>[2x]MNYWWVSQKQTFKQEFEGGYMWSPKENKNGTQSHYYNNMTLVQPGDVVFSFANGLILSVGIARSHAYSYNKPTEFGVAGADWANDGWKIDLEYHLVENKIRPKAHIDFIRPYLPQKYSPLQDNGNGNQAYLFSVPHELASKVVELIGSEAEEVIFGFADTTEITTTADAIECQISNDASIDETEKHQLVKSRRGQGIFRSRLEQVESRCRVTGVQLKNHLIASHIKPWAVSNNQERLDGHNGLLLAPHVD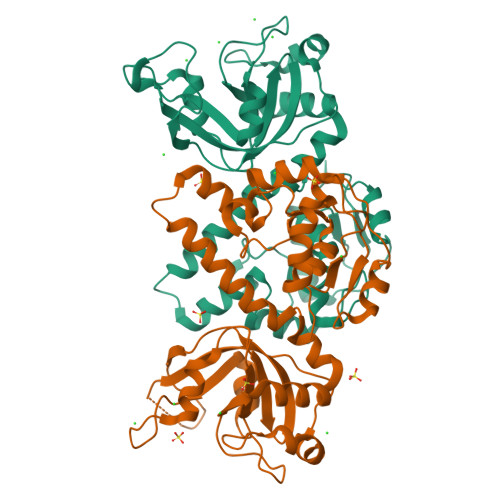HLFDKGFISFEDNGEMIVSEKLNLDVLKAWSISQGNYGYFSKQQQEYMCYHRENVFKKL> GHMSQHLPLVAAQPGIWMAEKLSELPSAWSVAHYVELTGEVDSPLLARAVVAGLAQADTLRMRFTEDNGEVWQWVDDALTFELPEIIDLRTNIDPHGTAQALMQADLQQDLRVDSGKPLVFHQLIQVADNRWYWYQRYHHLLVDGFSFPAITRQIANIYCTWLRGEPTPASPFTPFADVVEEYQQYRESEAWQRDAAFWAEQRRQLPPPASLSPAPLPGRSASADILRLKLEFTDGEFRQLATQLSGVQRTDLALALAALWLGRLCNRMDYAAGFIFMRRLGSAALTATGPVLNVLPLGIHIAAQETLPELATRLAAQLKKMRRHQRYDAEQIVRDSGRAAGDEPLFGPVLNIKVFDYQLDIPDVQAQTHTLATGPVNDLELALFPDVHGDLSIEILANKQRYDEPTLIQHAERLKMLIAQFAADPALLCGDVDIMLPGEYAQLAQLNATQVEIPETTLSALVAEQAAKTPDAPALADARYLFSYREMREQVVALANLLRERGVKPGDSVAVALPRSVFLTLALHAIVEAGAAWLPLDTGYPDDRLKMMLEDARPSLLITTDDQLPRFSDVPNLTSLCYNAPLTPQGSAPLQLSQPHHTAYIIFTSGSTGRPKGVMVGQTAIVNRLLWMQNHYPLTGEDVVAQKTPCSFDVSVWEFFWPFIAGAKLVMAEPEAHRDPLAMQQFFAEYGVTTTHFVPSMLAAFVASLTPQTARQSCATLKQVFCSGEALPADLCREWQQLTGAPLHNLYGPTEAAVDVSWYPAFGEELAQVRGSSVPIGYPVWNTGLRILDAMMHPVPPGVAGDLYLTGIQLAQGYLGRPDLTASRFIADPFAPGERMYRTGDVARWLDNGAVEYLGRSDDQLKIRGQRIELGEIDRVMQALPDVEQAVTHACVINQAAATGGDARQLVGYLVSQSGLPLDTSALQAQLRETLPPHMVPVVLLQLPQLPLSANGKLDRKALPLPELKAQAPGRAPKAGSETIIAAAFSSLLGCDVQDADADFFALGGHSLLAMKLAAQLSRQVARQVTPGQVMVASTVAKLATIIDAEEDSTRRMGFETILPLREGNGPTLFCFHPASGFAWQFSVLSRYLDPQWSIIGIQSPRPNGPMQTAANLDEVCEAHLATLLEQQ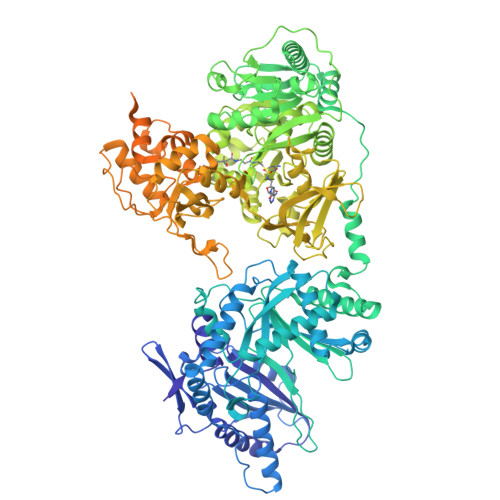PHGPYYLLGYSLGGTLAQGIAARLRARGEQVAFLGLLDTWPPETQNWQEKEANGLDPEVLAEINREREAFLAAQQGSTSTELFTTIEGNYADAVRLLTTAHSVPFDGKATLFVAERTLQEGMSPERAWSPWIAELDIYRQDCAHVDIISPGTFEKIGPIIRATLNR> ISGGDAIYSSTGRCSLGFNVRSGSTYYFLTAGHCTDGATTWWANSARTTVLGTTSGSSFPNNDYGIVRYTNTTIPKDGTVGGQDITSAANATVGMAVTRRGSTTGTHSGSVTALNATVNYGGGDVVYGMIRTNVCAEPGDSGGPLYSGTRAIGLTSGGSGNCSSGGTTFFQPVT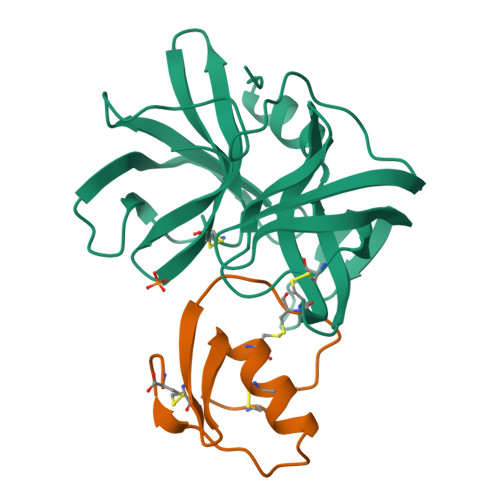EALVAYGVSVY;> VDCSEYPKPACTLEYRPLCGSDNKTYGNKCNFCNAVVESNGTLTLSHFGKC>MSAKSRTIGIIGAPFSKGQPRGGVEEGPTVLRKAGLLEKLKEQECDVKDYGDLPFADIPNDSPFQIVKNPRSVGKASEQLAGKVAEVKKNGRISLVLGGDHSLAIGSISGHARVHPDLGVIWVDAHTDINTPLTTTSGNLHGQPVSFLLKELKGKIPDVPGFSWVTPCISAKDIVYIGLRDVNPGEHYILKTLGIKYFSMTEVDRLGIGKVMEETLSYLLGRKKRPIHLSFDVDGLDPSFTPATGTPVVGGLTYREGLYITEEIYKTGLLSGLDIMEVNPSLGKTPEEVTRT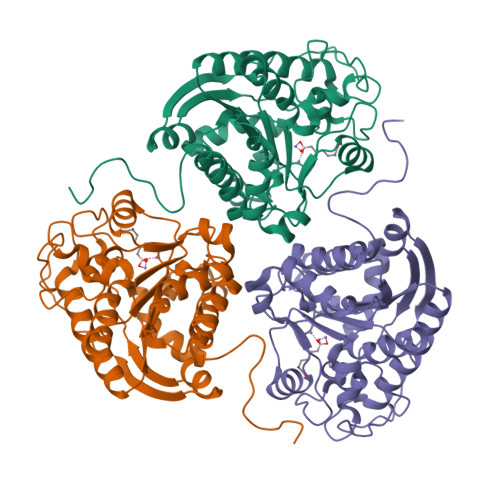VNTAVAITLACFGLAREGNHKPIDYLNPPK[2x]>NSSLDQIDLLSTKSFPPCMRQLHKALRENHHLRHGGRMQYGLFLKGIGLTLEQALQFWKQEFIKGKMDPDK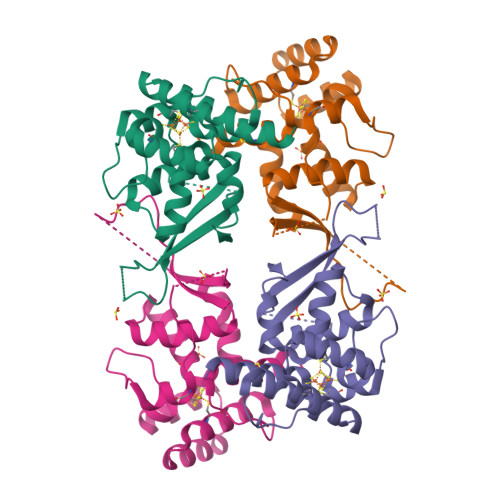FDKGYSYNIRHSFGKEGKRTDYTPFSCLKIILSNPPSQGDYHGCPFRHSDPELLKQKLQSYKISPGGISQILDLVKGTHYQVACQKYFEMIHNVDDCGFSLNHPNQFFCESQRILNGGKDIKKE[2x]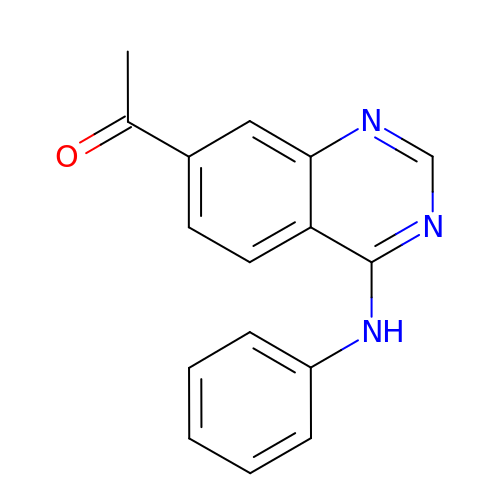1-(4-phenylazanylquinazolin-7-yl)ethanone | C16 H13 N3 O | PJPNKKKIJHLRQY-UHFFFAOYSA-N>[2x]GPLGSKIASAREVIKRDGVIP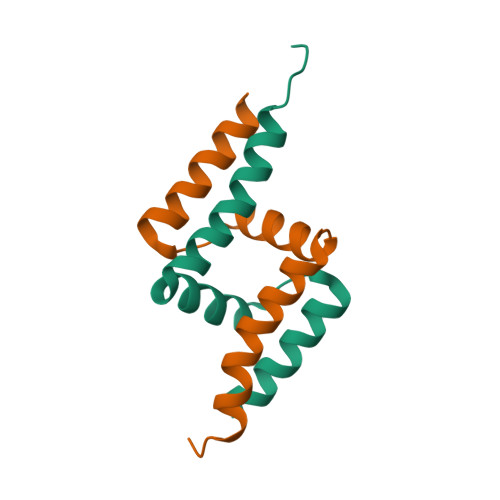PEALTIIEQRLRSDPMFRQQIDNVLADAECDANRAAYSP> MASEKHFKYVILGGGVAAGYAAREFAKQGVKPGELAIISKEAVAPYERPALSKGYLFPQNAARLPGFHVCVGSGGERQLPEWYSEKGIELILSTEIVKADLSTKTLTSAAGATFTYEILIIATGSSVIKLTDFGTQGADSNNILYLREIDDADKLVAAIQAKKGGKAVVVGGGYIGLELSAALKINDFDVTMVFPE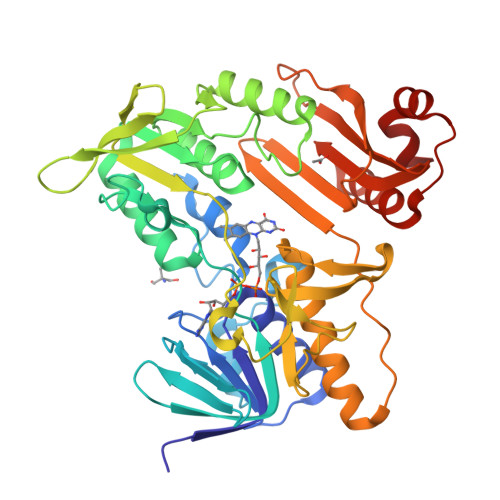PWCMPRLFTADIAAFYEAYYTNKGVKVLKGTLAVGFDANANGDVTAVKLKDGKVLEADIVVVGVGGRPLTTLFKGQVAEEKGGIKTDAFFETSVPGVYAIGDVATFPLKMYNELRRVEHVDHSRKSAEQAVKAIKGKESGESVPEYDYLPYFYSRSFDLGWQFYGDNVGETILFGDSDPTSSKPKFGSYWIKDGKVFGAFLEGGSPDENNAIAKVAKTQPPVASIEELKKEGLQFASKI>D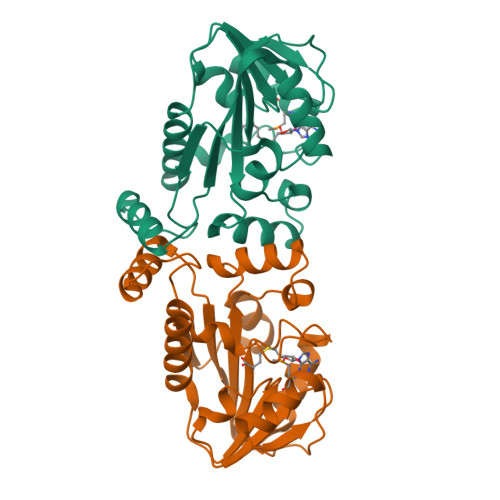PFASLAEAYEAWYGTPLGAYVIAEEERALKGLLPPGESLLEVGAGTGYWLRRLPYPQKVGVEPSEAMLAVGRRRAPEATWVRAWGEALPFPGESFDVVLLFTTLEFVEDVERVLLEARRVLRPGGALVVGVLEALSPWAALYRRLGEKGVLPWAQARFLAREDLKALLGPPEAEGEAVFLAPEAHPPYEEADLAGRRAGNRPALYLGRWR[2x]> AMKKDSKAPCVEVFDERDGCKAAGTQKASGDDGFCV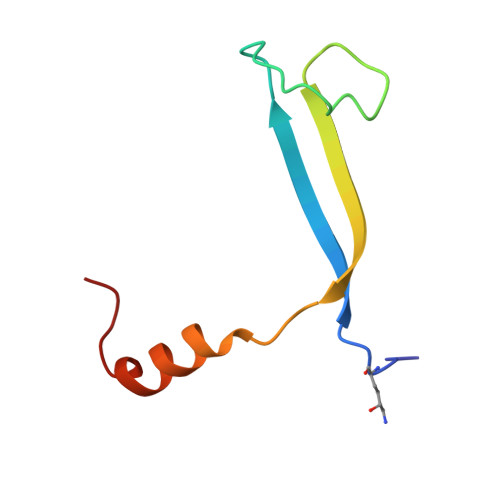KVSMKAIKMNAAEATSVTKNYNTKLL>SMTNNKYYTEENKKKVWKKHMIVLKFLEQPGISEAYLNYLQEEIHNDEWIGFENEFFEELTGKPVINVGDKIKATKQYSAVH[2x];>[2x]SMKRALGKAISYEEMAKGYEEMAAINSIIAQEDNHLENEAEMIKTRYKTLAS

Here we determined that the arbitrium system in Bacillus subtilis phage phi3T modulates the bacterial toxin–antitoxin system MazE–MazF to regulate the phage life cycle. AimX also inhibits the function of phi3T_93, a protein that promotes lysogeny by binding to MazE and releasing MazF. In all structures, phi3T_93 shows an identical all-helices fold composed of a longer N-terminal helix (α1), followed by two shorter helices (α2 and α3) connected by a long unstructured loop forming a V-like shape. The α1 helices of two phi3T_93 monomers interact, resulting in a W-shaped tight and globular dimer that displays two shallow grooves, one across each side of the dimer molecule.

The structure of the AimX–phi3T_93 complex showed that a phi3T_93 dimer binds two independent AimX molecules that are accommodated in the shallow grooves. Only a short fragment of AimX (residues 8–22; 30% of the protein), which folds as a 3-turn helix, is visible in the AimX–phi3T_93 crystal. The main contacts between AimX and phi3T_93 are nucleated by the projection of AimX M14 and M21 towards the hydrophobic bottom of the phi3T_93 groove generated by the side chains of K13, K17, W16, M20 and L23, pointing to these hydrophobic interactions as key for phi3T_93–AimX recognition. Additional polar and hydrophobic interactions stabilize the complex. The portion of AimX visible in the structure corresponds to an area of high sequence similarity with MazE and YosL, explaining why all these three proteins bind to MazF. Despite the structural differences between phi3T_93 (all alpha fold) and MazF (mainly beta fold), both AimX and MazE use an identical recognition mechanism by introducing a helix in the groove in the dimer’s interface. Structural alignment showed identical residues in the helix of AimX (M14, Y18, E20 and M21 for AimX) and MazE involved in the interactions with the corresponding partners, and YosLphi3T also presents identical residues in these positions. To test the potential binding partners of AimX, we used biolayer interferometry (BLI) assays, which showed that AimX does not bind to the master repressor phi3T_97 but binds to both MazF and phi3T_93. Interestingly, the affinity is more than twice as high for MazF than for phi3T_93. AimX can also bind to phi3T_93, preventing it from binding to MazE which would release MazF.> QEDEDGDYEELVLALRSE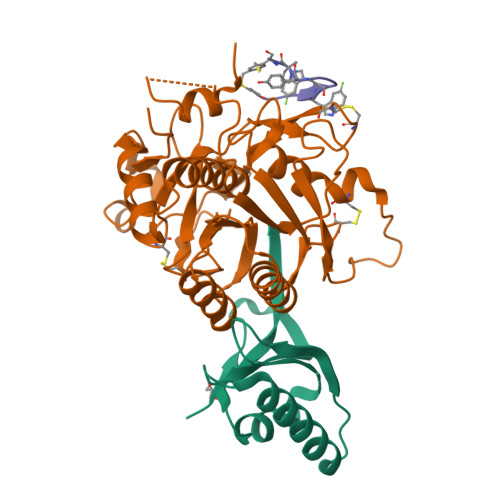EDGLAEAPEHGTTATFHRCAKDPWRLPGTYVVVLKEETHLSQSERTARRLQAQAARRGYLTKILHVFHGLLPGFLVKMSGDLLELALKLPHVDYIEEDSSVFAQ;> SIPWNLERITPPRYRADEYQPPDGGSLVEVYLLDTSIQSDHREIEGRVMVTDFENVPEEDGTRFHRQASKCDSHGTHLAGVVSGRDAGVAKGASMRSLRVLNCQGKGTVSGTLIGLEFIRKSQLVQPVGPLVVLLPLAGGYSRVLNAACQRLARAGVVLVTAAGNFRDDACLYSPASAPEVITVGATNAQDQPVTLGTLGTNFGRCVDLFAPGEDIIGASSDCSTCFVSQSGTSQAAAHVAGIAAMMLSAEPELTLAELRQRLIHFSAKDVINEAWFPEDQRVLTPNLVAALPPSTHGAGNSHHHHHH;> XKGWWDHYXCA3-[3-[3-[(4~{S})-6-azanyl-5-cyano-3-methyl-4-propan-2-yl-2~{H}-pyrano[2,3-c]pyrazol-4-yl]-5-(trifluoromethyl)phenyl]phenyl]propanoic 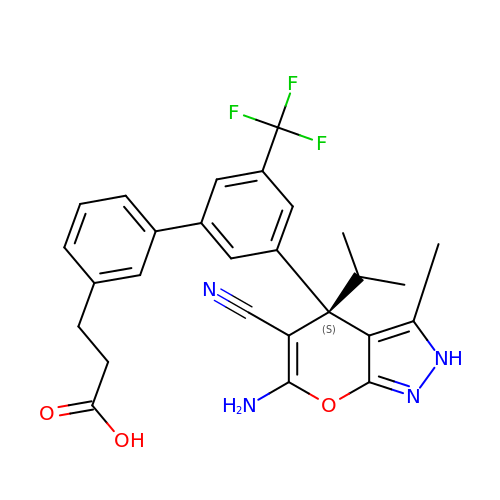acid | C27 H25 F3 N4 O3 | ULXPNGMLUPLOIA-SANMLTNESA-N4-(CARBOXYVIN-2-YL)PHENYLBORONIC ACID | C9 H9 B O4 | 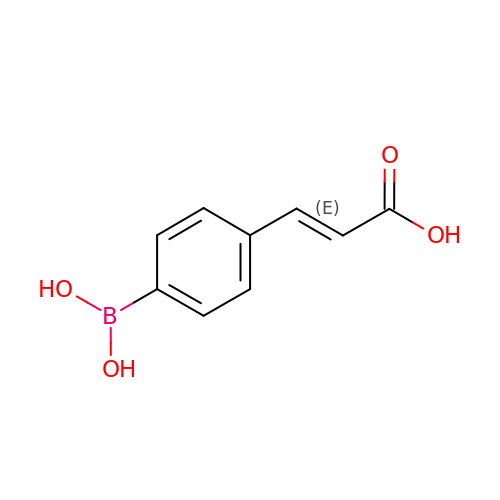IEMLKNHGGSYOMP-ZZXKWVIFSA-N> AVKRRPRFPVNSNSNGGNELCPKIRIGQDDLPGFDLISQFQVDKAASRRAIQRVVGSATLQVAYKLGNNVDFRIPTRNLYPSGLPEEYSFLTTFRMTGSTLKKNWNIWQIQDSSGKEQVGIKINGQTQSVVFSYKGLDGSLQTAAFSNLSSLFDSQWHKIMIGVERSSATLFVDCNRIESLPIKPRGPIDIDGFAVLGKLADNPQVSVPFELQWMLIHCDPLRPRRETCHE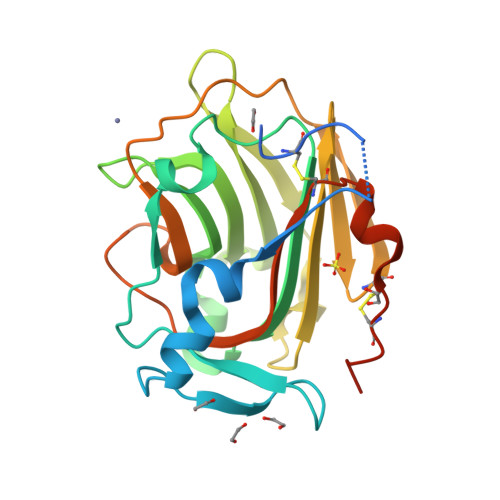LPARITPSQTTDER Typhoid toxin is an A2B5 protein toxin and an important virulence factor for the human-adapted bacterial pathogen Salmonella enterica serovar Typhi, the causative agent of typhoid fever. Typhoid toxin contains two enzymatic subunits, PltA and CdtB, which dock onto a pentameric delivery platform composed of the protein PltB. It was recently reported that the same enzymatic subunits can assemble with a different delivery platform composed of the protein PltC, forming a distinct version of typhoid toxin. Here, we determined atomic-level structures of the pentameric PltC subunit, the fully assembled PltC typhoid toxin, and the PltC pentamers in complex with glycan receptors.

The ligand-bound atomic structures of PltC show an additional glycan binding site not found in PltB and glycan array analysis indicates that PltB and PltC exhibit significant differences in glycan binding specificity. In contrast, we observed that PltC binds both Neu5Ac- and Neu5Gc-terminated glycans and did not demonstrate a clear preference between the two sialic acids. Strikingly, however, PltC showed much greater affinity for the Neu5Gc glycan than its Neu5Ac-terminated counterpart, whereas the binding of PltB to the Neu5Gc derivative was almost undetectable. As has been observed previously for PltB and ArtB, the structures of the apo and the glycan-bound forms of PltC are overall quite similar, indicating that glycan binding does not trigger large-scale conformational changes. Both structures reveal that each PltC monomer displays the canonical lateral side glycan-binding site observed in other homologous B subunits, including PltB. However, Tyr103 from PltC, which is absent in PltB, forms a direct hydrogen bond with the extra hydroxyl group of Neu5Gc and provides a structural basis for PltC to bind both Neu5Ac- and Neu5Gc-terminated glycans. Importantly, in addition to the lateral site, each PltC monomer has a second glycan-binding site located at the basal side of the protein (opposite from the face that interacts with PltA), which is formed by an additional spoon-like structure that is absent from PltB but which has also been observed in ArtB. The most critical residue within the second binding site is Ser45, which makes multiple contacts with both glycans and also stabilizes the extra hydroxyl group of the Neu5Gc-terminated glycan. Binding to different glycan receptors does not result in marked conformational changes in PltC. In accordance with the results above, we found that the S31A mutant exhibited binding affinities similar to that of wild-type PltC, whereas the binding affinities of the S45A mutant were drastically reduced and similar to those of the S31A/S45A double mutant. Together, these results indicate that PltC’s glycan binding specificity is largely mediated by a second glycan binding site not found in PltB, which is likely a key determinant of the different trafficking and cell targeting properties observed for the two typhoid toxins.

>[5x]AMADYDTYVSNVQINNLSYGVYTSGGKETQFFCIGLKHGSEAISINAMCKVDVYGNHKQGFDNMLNTAKYYYTTGGDVRIYYKENVWRDPDFKSAFSSRELIAITTCSSSSYCMGPTVTNLESD> HMMDMTQQEIFDKQRRLQELSEKVRTCHQEISALRKALQEKEAEMLQVL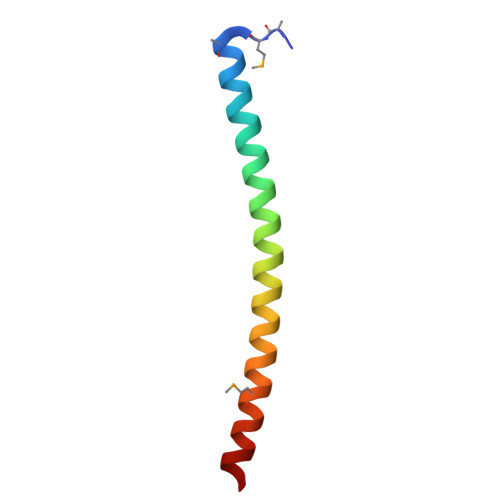EDIQTI3-[(3'-AMINOMETHYL-BIPHENYL-4-CARBONYL)-AMINO]-2-(3-CARBAMIMIDOYL-BENZYL)-BUTYRIC ACID 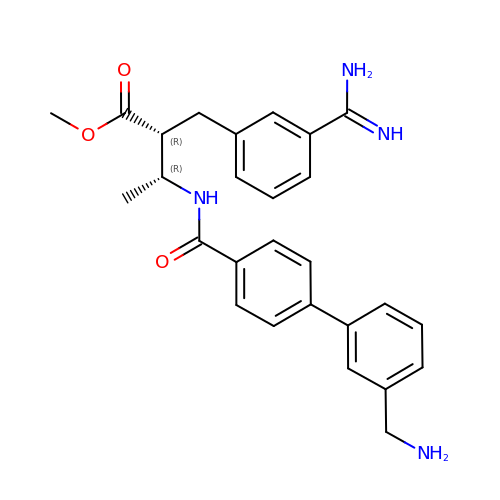METHYL ESTER | C27 H30 N4 O3 | XFKVLKLCLYJKNF-MZNJEOGPSA-N> MEALEELMKLLNMKDFPYRIEGIDISHLQGKYTVASLVVFEDGFPKKGDYRRYKIEQDHPDDYESIRTVVKRRYSKHPLPNLLFVDGGIGQVNAAIEALKEIGKDCPVVGLAKKEETVVFENREIHLPHDHPVLRLLVQIRDETHRFAVSYHRKRRE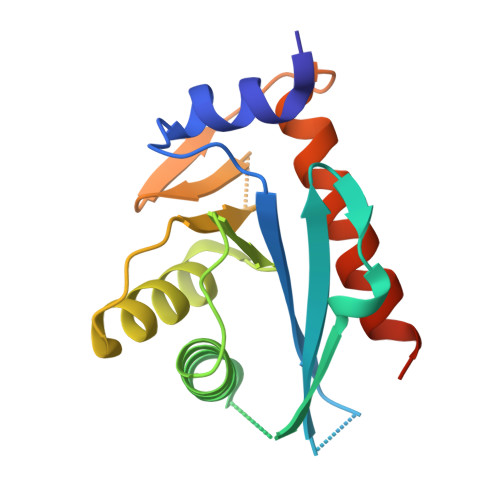KE>GSHMSKSALVILAPGAEEMEFIIAADVLRRAGIKVTVAGLNGGEAVKCSRDVQILPDTSLAQVASDKFDVVVLPGGLGGSNAMGESSLVGDLLRSQESGGGLIAAICAAPTVLAKHGVASGKSLTSYPSMKPQLVNNYSYVDDKTVVKDGNLITSRGPGTAYEFALKIA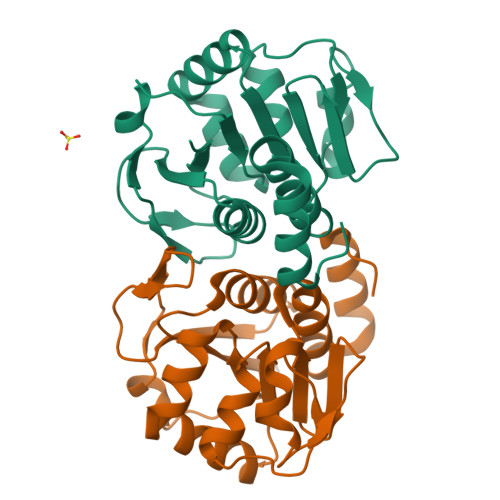EELAGKEKVQEVAKGLLVAYN[2x]>[8x]AMITGGELVVRTLIKAGVEHLFGLHGIHIDTIFQACLDHDVPIIDTRHEAAAGHAAEGYARAGAKLGVALVTAGGGFTNAVTPIANAWLDRTPVLFLTGSGALRDDETNTLQAGIDQVAMAAPITKWAHRVMATEHIPRLVMQAIRAALSAPRGPVLLDLPWDILMNQIDEDSVIIPDLVLSAHGARPDPADLDQALALLRKAERPVIVLGSEASRTARKTALSAFVAATGVPVFADYEGLSMLSGLPDAMR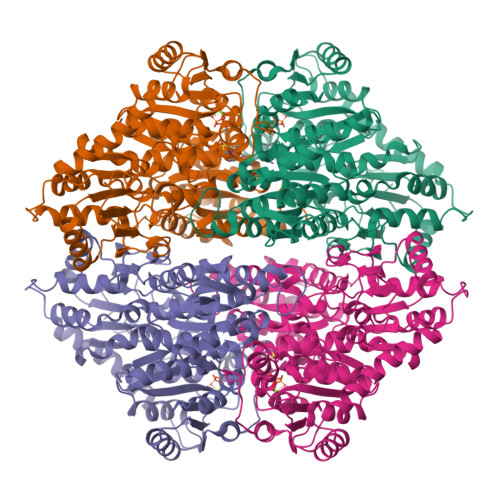GGLVQNLYSFAKADAAPDLVLMLGARFGLNTGHGSGQLIPHSAQVIQVDPDACELGRLQGIALGIVADVGGTIEALAQATAQDAAWPDRGDWCAKVTDLAQERYASIAAKSSSEHALHPFHASQVIAKHVDAGVTVVADGGLTYLWLSEVMSRVKPGGFLCHGYLNSMGVGFGTALGAQVADLEAGRRTILVTGDGSVGYSIGEFDTLVRKQLPLIVIIMNNQSWGWTLHFQQLAVGPNRVTGTRLENGSYHGVAAAFGADGYHVDSVESFSAALAQALAHNRPACINVAVALDPIPPEELILIGMDPFAGSTENLYFQSGALEHHHHHH>[2x]MELLWCELNRDLPTPLYEQLYAHIKTEITEGRIGYGTKLPSKRKLADSLKLSQNTVEAAYEQLVAEGYVEVIPRKGFYVQAYEDLEYIRAPQAPGDALATKQDTIRYNFHPTHIDTTSFPFEQWRKYFKQTMCKENHRLLLNGDHQGEASFRREIAYYLHHSRGVNCTPEQVV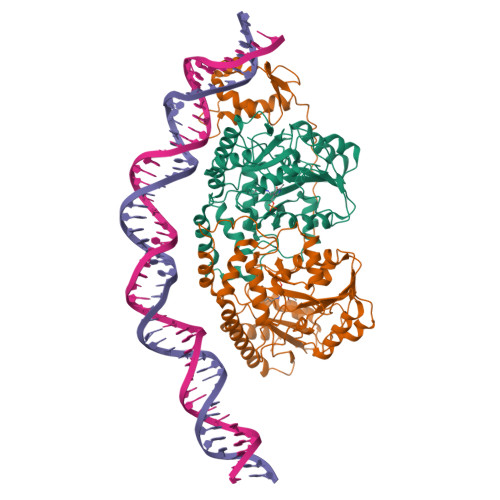VGAGVETLLQQLFLLLGESKVYGIEDPGYQLMRKLLSHYPNDYVPFQVDEEGIDVDSIVRTAVDVVYTTPSRHFPYGSVLSINRRKQLLHWAEAHENRYIIEDDYDSEFRYTGKTIPSLQSMDVHNKVIYLGAFSKSLIPSVRISYMVLPAPLAHLYKNKFSYYHSTVSRIDQQVLTAFMKQGDFEKHLNRMRKIYRRKLEKVLSLLKRYEDKLLIIGERSGLHIVLVVKNGMDEQTLVEKALAAKAKVYPLSAYSLERAIHPPQIVLGFGSIPEDELEEAIATVLNAWGFLVPRGSLEHHHHHH> MEHVPAELTRVSEGYTRFYRSPTASVILSGLVKVKWDNEQMTMPLFKWIGGEQAEELHFCVHIAHSSGPKLNRA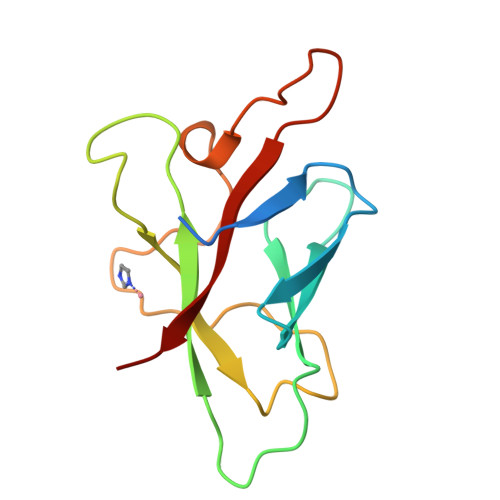RSLGTVNSNMDQHWAQAQRNSGATRRTIEGFHLFENDIPNFPDYIKIKLVPKT>[2x]SNAYTPALNRPLLLNNYKESQRRLFLFDYDGTLTPIVQDPAAAIPSDKLNRILDVLSSDPKNQIWIISGRDQAFLEKWMGNKNVGLSAEHGCFMKDIGSKEWVNLAASFDMSWQEKVDDIFKYYTEKTPG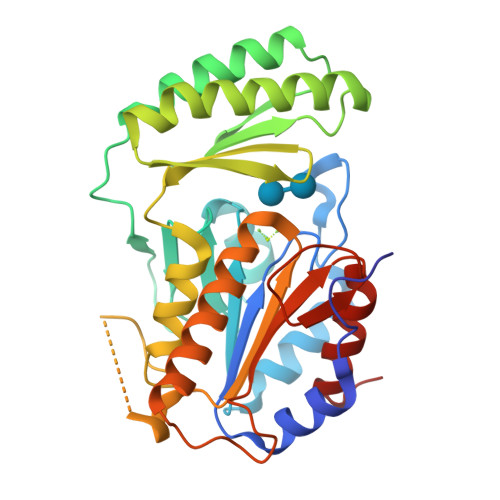SNIERKKVALTWHYRRADPDLGNFQAEKCMKELNDTVAKEYDVEVMAGKANIEVRPKFVNKGEIVKRLVLHPHGAKQEKHPTGHCTKDIPIEELPDFMLCLGDDLTDEDMFNSLNEINKKWKGDNRPTNKFGSYGVYPVAVGPASKKTVAIAHLNEPRQVLETLGLLAGLVS>[2x]SLPACPEESPLLVGPMLIEFNMPVDLELVAKQNPNVKMGGRYAPRDCVSPHKVAIIIPFRNRQEHLKYWLYYLHPV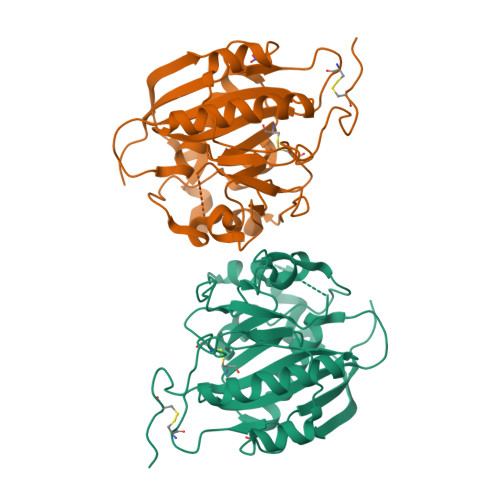LQRQQLDYGIYVINQAGDTIFNRAKLLNVGFQEALKDYDYTCFVFSDVDLIPMNDHNAYRCFSQPRHISVAMDKFGFSLPYVQYFGGVSALSKQQFLTINGFPNNYWGWGGEDDDIFNRLVFRGMSISRPNAVVGRCRMIRHSRDKKNEPNPQRFDRIAHTKETMLSDGLNSLTYQVLDVQRYPLYTQITVDIGTPS>MSGRWSHPQFEKIHQRREAGARETCRDQIKGSDKDEEPSAALSHGQGYRPCGRPARNSKPEAGARPPAVPIMVNDPPVPALLWAQEVGHVLAGRARRLMLQFGVLFCTILLLLWVSVFLYGSFYYSYMPTVSHLSPVHFHYRTDCDSSTASLCSFPVANVSLAKSGRDRVLMYGQPYRVTLELELPESPVNQDLGMFLVTVSCYTRGGRIISTSSRSVMLHYRSQLLQVLDTLLFSSLLLFGFAEQKQLLEVELYSDYRENSYVPTTGAIIEIHSKRIQMYGAYLRIHAHFTGLRYLLYNFPMTCAFVGVASNFTFLSVIVLFSYMQWVWGAVWPRHRFSLQVNIRQRDNSHHGAPRRISRHQPGQESTQQSDVTEDGESPEDPSGTEGQLSEEEKPEKRPLNGEEEQEPEASDGSWEDAALLTEANPPTSASASALAPETLGSLRQRPTCSSS[12x];>MKYPLVPLVSDLTLSFLVFWLCLPV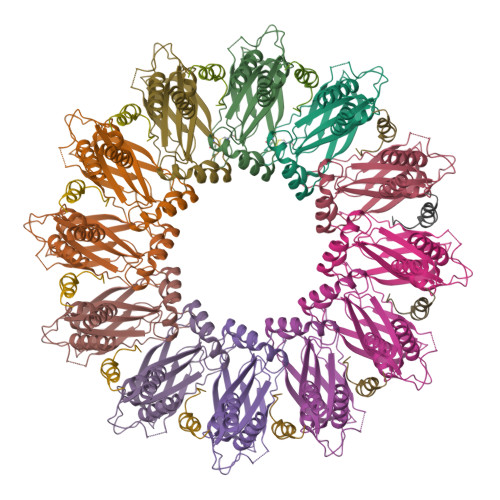ALLLFLTIVWLHFLLSQESKEDDSDLCFNWEPWSKRPSECGCEETFPGEEDGLHWGGSGSGDYKDDDDK[12x]>MGSSHHHHHHSQDPNSMKRLKDLREYLAVLEAHQDVREIDEPVDPHLEAGAAARWTYENRGPALMLNDLTGTGRFCRILAAPAGLSTIPGSPLARVALSLGLDVSATAHEIVDSLAAARTREPVAPVVVDSAPCQDNVLLGDDANLDRFPAPLLHEGDGGPYLNTWGTIIVSTPDGSFTNWAIARVMKIDGKRMTGTFIPTQHLGQIRKLWDNLGQPMPFAIVQGTEPGIPFVASMPLPDGIEEVGFLGAYFGEPLELVRAKTVDLLVPASAEIVIEGHVMPGRTAVEGPMGEYAGYQPRHTSMQPEYVVDAITYRDDPIWPISVAGEPVDETHTAWGLVTAAEALALLRAAKLPVATAWMPFEAAAHWLIVCLTEDWRERMPGLSRDGICLRISQVLAATRIEAMMTRVFVLDDDVDPSDQTELAWAIATRVS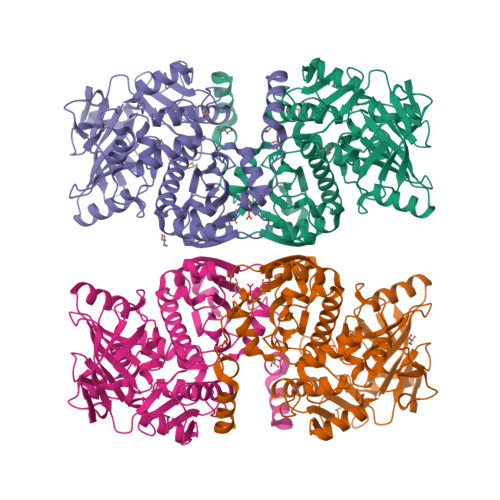PAHGRLVRHGMINPLAGCYSAEERRLGYGPKAVLNGLLPPMAERSRRSSFRHTYPEPVRQRVIELLA[4x]> MSLYKVYGDYRSGNCYKIKLMLNLLGLPYEWQAVDILGGDTQTEAFLAKNPNGKIPVLELEDGTCLWESNAILNFLADGSQFLPSEPRLRTQVLQWQFFEQYSHEPYIAVARFIQLYEGLPEERREEYLKLHKRGYKALDVMEKQLSRTPYLVGEHYSIADIALYAYTHVADEGGFDLSRYPGIQAWMQRVQSHPRHVPMLDEGHHH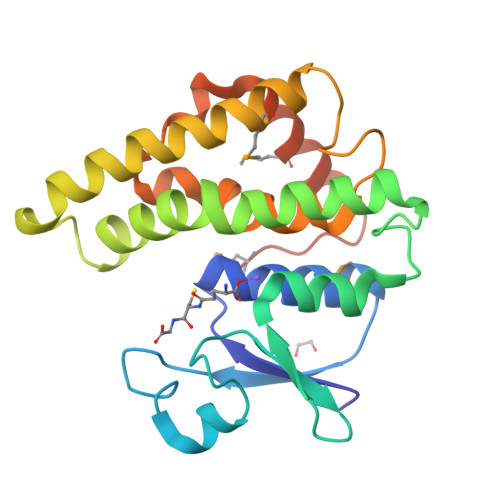HHH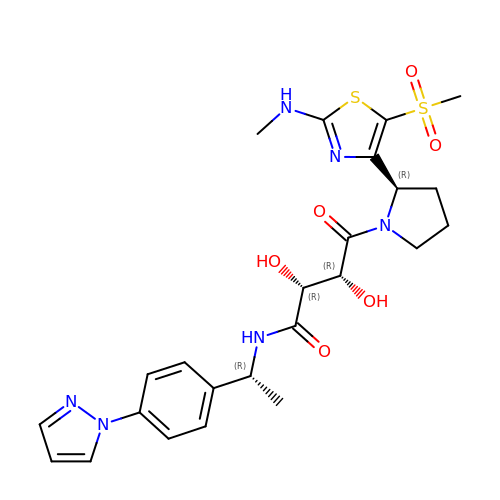(2R,3R)-2,3-dihydroxy-4-{(2R)-2-[2-(methylamino)-5-(methylsulfonyl)-1,3-thiazol-4-yl]pyrrolidin-1-yl}-4-oxo-N-{(1R)-1-[4-(1H-pyrazol-1-yl)phenyl]ethyl}butanamide | C24 H30 N6 O6 S2 | QFHBCQAIZQPRLF-SJFSSXKUSA-N> MSLFGNTTTGGGGLFGNTTTPTQTTGGGLFGNTTTGGGLFGNTATPTTGGGGLFGNTATPTLTTGGGGGLFGNTTAPTTGGGGLFGNTPTQTTGGGLFGNTATGGGGLFGNTQQQQQQQQQQQQQQQQQQQQQPSTSLFSQSSLGSQSSLGSQSSLGSQSSLGSQSSLGSFGQTQQPQTSSLFGNLQQQQQLQQPQRSIIEQKLYDFMQSISPNSLNCRFLYWFYNYQANGQLVDPNSIPKPPNVTVDQWAYALSNNPDPSILIPVAAKS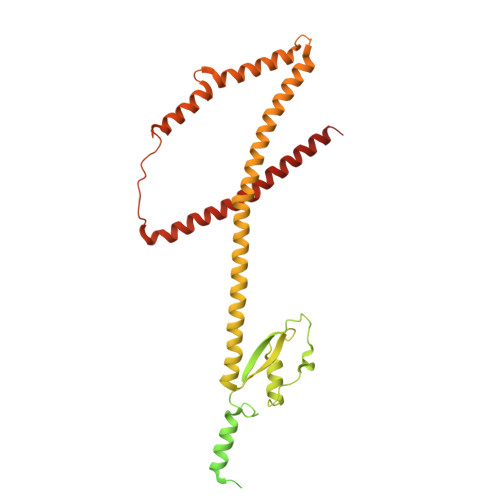FDDLINRRMKQEETIIALDQNTQEALKRMRDLENHLNFHIHTQLEMMRKKQIELIQRYIEVWSNLEIYQSKGKTFTTSEERIMKKIYELFEEINQPNSIKSKVEEISNQLKLGSMEKEKIKYEISPEAVEPLYNLLKNMTISIERITNELEIAVKDAQILKNELYQLKKC> LATKAARKSAPA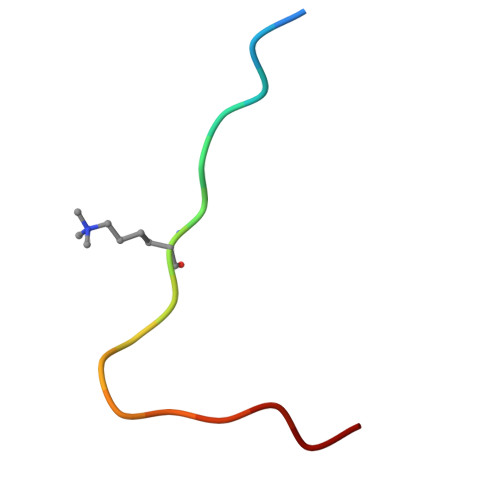TGGVK> RVPPPPPCCHPRLSLHRPALEDLLLGSEANLTCTLTGLRDASGATFTWTPSSGKSAVQGPPERDLCGCYSVSSVLPGSAQPWNHGETFTCTAAHPELKTPLTATLSKSGNTFRPEVHLLPPPSEELALNELVTLT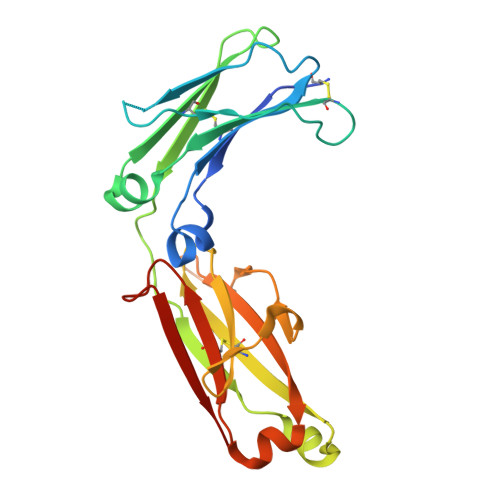CLARGFSPKDVLVRWLQGSQELPREKYLTWASRQEPSQGTTTFFVYSILRVAAEDWKKGDTFSCMVGHEALPLAFTQKTIDRLAG> ATGDERFYAEHLMPTLQGLLDPESAHRLAVRFTSLGLLPRARFQDSDMLEVRVLGHKFRNPVGIAAGFDKHGEAVDGLYKMGFGFVEIGSVTPKPQEGNPRPRVFRLPEDQAVINRYGFNSHGLSVVEHRLRARQQKQAKLTEDGLPLGVNLGKNKTSVDAAEDYAEGVRVLGPLADYLVVNVSSPNTAGLRSLQGKAELRRLLTKVLQERDGLRRVHRPAVLVKIAPDLTSQDKEDIASVVKELGIDGLIVTNTTVSRPAGLQGALRSETGGLSGKPLRDLSTQTIREMYALTQGRVPIIGVGGVSSGQDALE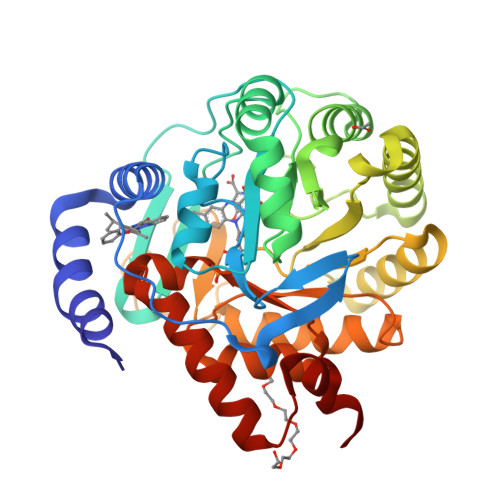KIRAGASLVQLYTALTFWGPPVVGKVKRELEALLKEQGFGGVTDAIGADHRR> SNIQTGAERMPHDLSHLGFLAGQIGRLITISTTPVIAGDSFEMDAVGALRLSPLRRGLAIDSTVDIFTFYVPHRHVYGEQWIKFMKDGVNATPLPTVNTTGYIDHAAFLGTINPDTNKIPKHLFQGYLNIYNNYFKAPWMPDRTEANPNELNQDDARYGFRCCHLKNIWTAPLPPETELSRQMTTSTTSIDIMGLQAAYANLHTDQERDYFMQRYRDVISSFGGKTS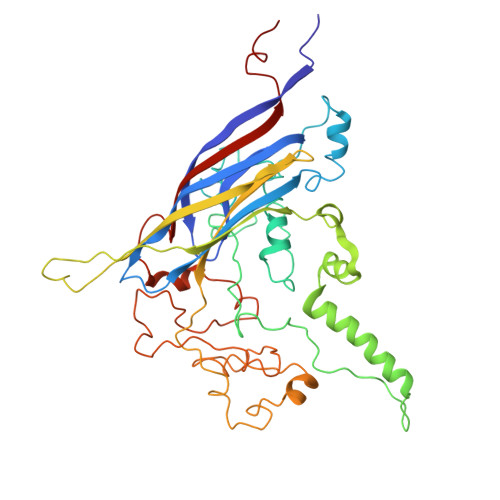YDADNRPLLVMRSNLWASGYDVDGTDQTSLGQFSGRVQQTYKHSVPRFFVPEHGTMFTLALVRFPPTATKEIQYLNAKGALTYTDIAGDPVLYGNLPPREISMKDVFRSGDSSKKFKIAEGQWYRYAPSYVSPAYHLLEGFPFIQEPPSGDLQERVLIRHHDYDQCFQSVQLLQWNSQVKFNVTVYRNLPTTRDSIMTS> NTFEDFYLKRELLMGIFEAGFEKPSPIQEEAIPVAITGRDILARAKNGTGKTAAFVIPTLEKVKPKLNKIQALIMVPTRELALQTSQVVRTLGKHCGISCMVTTGGTNLRDDILRLNETVHILVGTPGRVLDLASRKVADLSDCSLFIMDEADKMLSRDFKTIIEQILSFLPPTHQSLLFSATFPLTVDEFMDKHLHKPYEINLMEE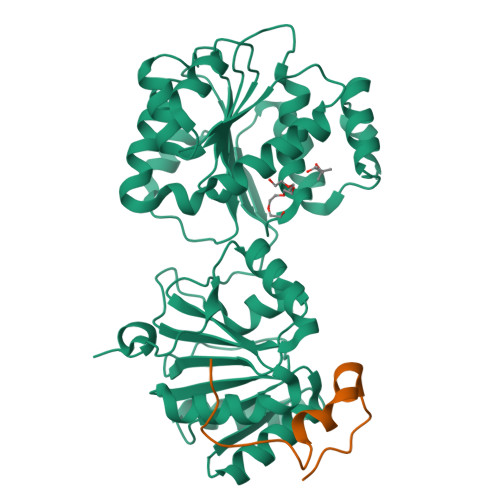LTLKGITQYYAFVEERQKLHCLNTLFSKLQINQAIIFCNSTNRVELLAKKITDLGYSCYYSHARMKQQERNKVFHEFRQGKVRTLVCSDLLTRGIDIQAVNVVINFDFPKTAETYLHRIGRSGRFGHLGLAINLINWNDRFNLYKIEQELGTEIAAIPATIDKSLYVAEN;> GLENSGNARDGPLDFEESYKGYGEHELEENDYLNDETFGDNVQVGTDFDFGNPHSSGSSGNAIGGNGVGATARSY>[2x]MASGMTVTDAGADQPIVFVNRAFSTITGYAPNEVLGRNARFLQG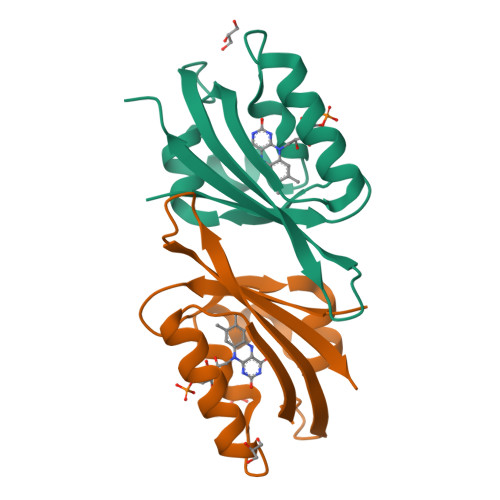PQTDAATVARLREAIAAARPIQERILNYRKDGQPFWNQLSISPVRDETGNVVAFVGVKTDVTAHHHHHH> GAMAMPALPLDQLQITHKDPKTGKLRTSPALHPEQKADRYFVLYKPPPKDNIPALVEEYLERATFVANDLDWLLALPHDKFWCQVIFDETLQKCLDSYLRYVPRKFDEGVASAPEVVDMQKRLHRSVFLTFLRMSTHKESKDHFISPSAFGEILYNNFLFDIPKILDLCVLFGKGNSPLLQKMIGNIFTQQPSYYSDLDETLPTILQVFSNILQHCGLQGDGANTTPQKLEERGRLTPSDMPLLELKDIVLYLCDTCTTLWAFLDIFPLACQTFQKHDFCYRLASFYEAAIPEMESAIKKRRLEDSKLLGDLWQRLSHSRKKLMEIFHIILNQICLLPILESSCDNIQGFIEEFLQIFSSLLQEKRFLRDYDAL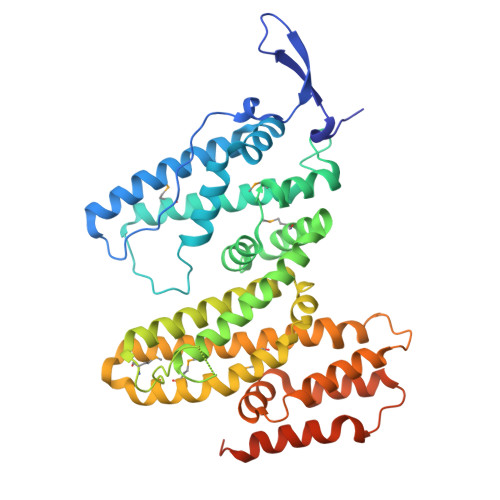FPVAEDISLLQQASSVLDETRTAYILQAVESAWEGVDRRKATDAKDPSVIEEPNGEPNGVTVTA> M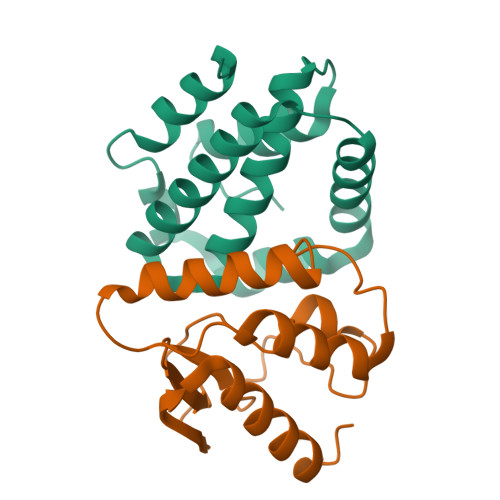INNKLIEIDNCLSAPSFFDFLKSLNVDSALDSRDEPEFDDCWMSEFNSLDKESFQDDDIEFIDSLREKAFKYSFRVINNAEISSRISDDIEIISKSFVLEKENSWSITHLWSSYKNGKFPE;> GSSHHHHHHENLYFQGMGVSESGHHVPAVRKSKGRPFEVSRFDKTRPTLFPRGENPEHSAWRLHHAERDVIGPRQGDFPGSDKELFDAYRKAYSKLDDIRVDVKSPNGTYTLGTNVTPSKAVDLIEVWLKGQGLM> MITGYSTPSAHVLMSSRAFKSSSYRA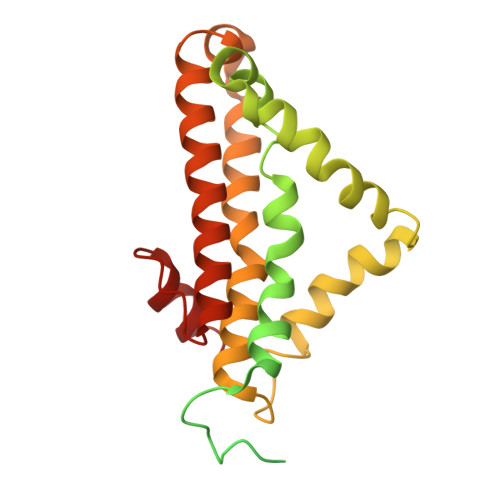AAGQTQHYLARSSLPVVKNSWGSPPSPFNELPRVSRGVPLSYLSASSSLLLNGEQGSLSGTLPVLPVRRKTLLTPRASKDVPSSFRFPPMTKKPQWWWRTLACLPYLMPLHETWMYAETAYHLHPFLEDFEFLTYPFLGAIGRLPSWFLMAYFFVAYLGIVRRKEWPHFFRFHVVMGMLLEIALQVIGTVSKWMPLGVYWGKFGMHFWTAVAFAYLFTVLESIRCALAGMYADIPFVCDAAYIQIPYD> MGIPLTPLFSRYKDSYLLYSFRLIDLLRASKSTHLTKLLSSQATYLYHFACLMKYKDIQKYEVQQLIEWAINASPDMDLQQFRIEFMDKTTELNLRSCQPKSFTYTFTTIWDTMHFLSLIIDDMVYTRDKSSLDFVMQQLKTMKVLFYNVFFILQCAMCRDHYMNVKGFIIYHIELIEIALDKEKYGTDITFVDSYQQETAGA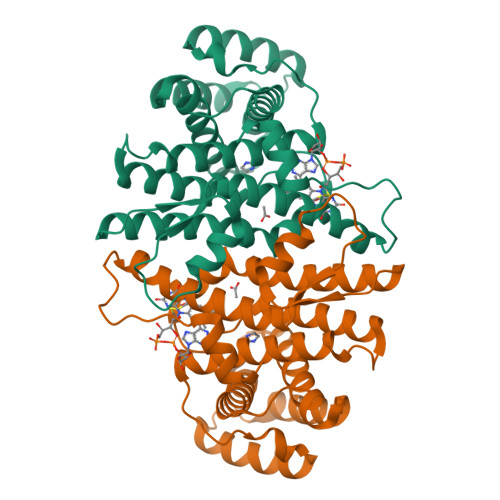DVAVVSNNMLMKNLMAYVSMTFHNHINDYKWIQRNKKPPAHYERMTWGEYKKLLNLQQLVPRG> RNCSSNEERKRRKYFHMLYLVCLMVHGFIRNEWINSKRLSRKLSNLVPEKVFELLHPQKDEELPLRS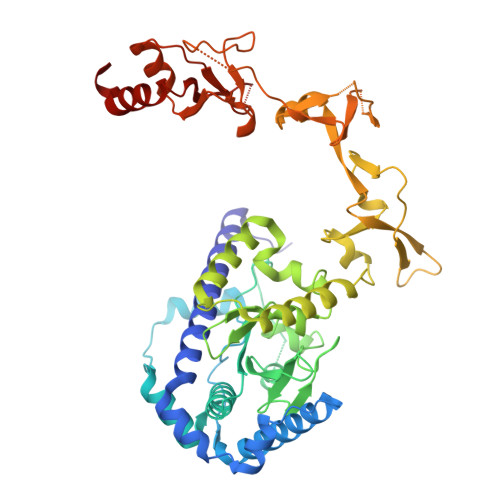TRKLLDGLKKCMELWQKHWKITKKYDNEGLYMRTWKEIEMSANNKRKFKTLKRSDFLRAVSKGHGDPDISVQGFVAMLRACNVNARLIMSCQPPDFTNMKIDTSLNGNNAYKDMVKYPIFWCEVWDKFSKKWITVDPVNLKTIEQVRLHSKLAPKGVACCERNMLRYVIAYDRKYGCRDVTRRYAQWMNSKVRKRRITKDDFGEKWFRKVITALHHRKRTKIDDYEDQYFFRRDESEGIPDSVQDLKNHPYYVLEQDIKQTQIVKPGCKECGYLKVHGKVGKVLKVYAKRDIADLKSARQWYMNGRILKTGSRCKKVIKRTVGRPKGEAEEDAERLYSFEDTELYIPPLASASGEITKNTFGNIEVFAPTMIPGNCCLVENPVAIKAARFLGVEFAPAVTSFKFERGSTVKPVLSGIVVAKWLREAIETAIDGIEFI> MLMRTDPFRDLDRFAQQVLGTSARPAVMPMDAWREGDKFVVEFDLPG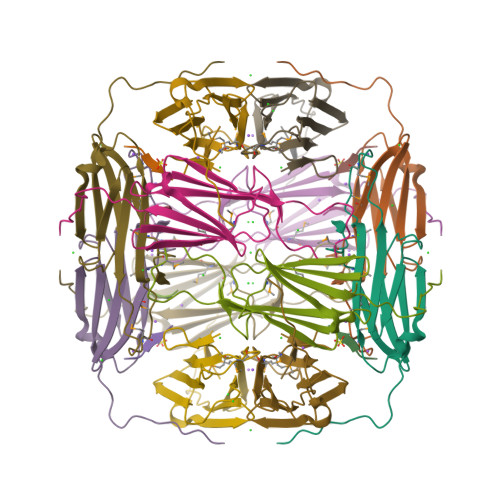IDADSLDIDIERNVVTVRAERPAVDPNREMLASERPRGVFSRQLVLGENLDTARIAASYTEGVLKLQIPVAEKAKPRKISITRGAGDKTISENGAHPEVIEA;> GRLLP> SKYSSSFGRLRR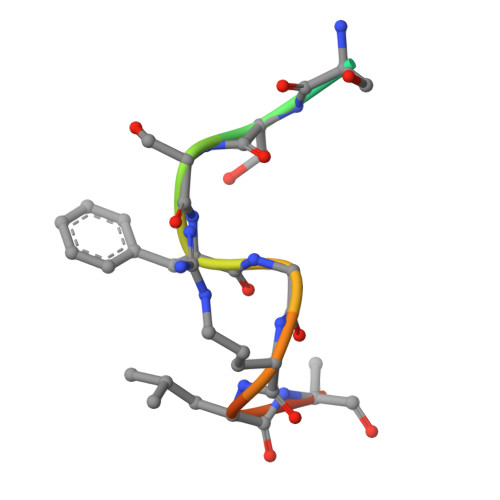Q> MDKRRVVVTGIGAVTPIGNDAETSWENAKKGVNGVAKMTRLNPDDFPVKIAAELKDFDVEKYLEKKEARKMDRFTHYAIASAEMAVQDSGLVIDDSNANRVGVWIGSGIGGMETFETQYEIFLNRGHRRVSPFFVPMMIPDMGSGQVSIRFGAKGINSTTVTACATATNSIGDAFKVIERGDADAMITGGAEAPITKMSLAGFTANKALSLNPDPETACRPFDKDRDGFIIGEGAGIVILEEYEHAKARGAKIYAEIVGYGATGDAYHITAPAPNGEGAARAMKMAIDDAGLTPDK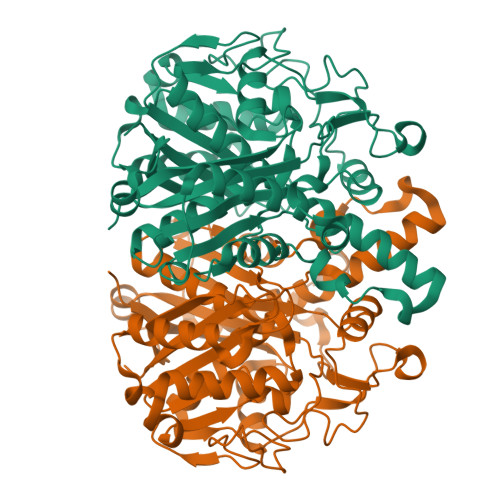VDYINAHGTSTPYNDEYETQAIKTVFGDHAKKLAISSTKSMTGHTLGASGGIEAIFALLTIRDNIIAPTIHLKNQDEVCDLDYVPNEAREANVNVVISNSFGFGGHNATLVFKRIED> MHHHHHHIFPKQYPIINFTTAGATVQSYTNFIRAVRGRLTTGADVRHEIPVLPNRVGLPINQRFILVELSNHAELSVTLALDVTNAYVVGYRAGNSAYFFHPDNQEDAEAITHLFTDVQNRYTFAFGGNYDRLEQLAGNLRENIELGNGPLEEAISALYYYSTGGTQLPTLARSFIICIQMISEAARFQYIEGEMRTRIRYNRRSAPDPSVITLENSWGRLSTAIQESNQGAFASPIQLQRRNGSKFSVYDVSILIPIIALMVYRCAPPPSSQF

Ricin is an AB toxin consisting of an enzymatically active A subunit (Ricin Toxin A-chain, RTA) and a cell-binding B subunit (Ricin Toxin B-chain, RTB) linked by a disulfide bond. RTA is highly catalytically active in depurinating the adenine base at position 4324 (A4324) selectively in a specific region in the 28S rRNA to inhibit ribosomal protein biosynthesis, causing cell death. The active site of RTA consists of two pockets, the primary pocket catalyzing the depurination of A4324 and the secondary pocket accommodating the guanine residue adjacent to A4324, with Tyr80 dividing these pockets. Thus, in this study, we report the synthesis of 7PCAs with tripeptide pendants having elongated C-terminal residues, in which ornithine and lysine residues with an aromatic ring were employed as the C-terminal residues to direct the interaction with the secondary pocket.

Co-crystals of RTA with 4a and 4b were prepared using the hanging drop vapor diffusion crystallization method and their crystal structures were analyzed. In each case, the pterin ring interacted with Gly121, Asn122, Tyr123, Ile172, and Arg180 in the primary pocket of RTA through the same interactions as those previously observed with other pterin derivatives. For 4a, the tripeptide moiety was unsuccessfully assigned, probably because only the pterin moiety was accommodated in the primary pocket and the pendant moiety was free to move. For 4A, the displacement of Tyr80, as well as the T-shaped interactions, were not observed, even though it had the same P1-P2 moiety, Gly-Phe. It is likely that the alkyl chain of the C-terminal residue in 4A is not long enough to form the hydrogen bonds with the residues at the entrance of the secondary pocket; consequently, the unfixed large side chain is free to move, preventing the phenyl ring in P2 from forming a T-shape interaction. The same movements of Tyr80 were observed in the crystal structures of RTA with the potent inhibitors 1, 2, while no such conformational change was observed in RTA crystals with 4a and other low-activity inhibitors such as 3, for which the positions of Tyr80 was the same as in the inhibitor-free crystal structure. Compound 4b exhibited an IC50 value of 33.4±2.7 μM, whereas compound 4a exhibited an IC50 value of 485±33 μM. The weak inhibitory activity of 4a was comparable to that of pterin-7-carboxylic acid, which is consistent with the fact that only the pterin-7-carboxylic acid portion was assigned in the X-ray crystallography of 4a/RTA and no conformational change in Tyr80 was observed.>ADLGSPCGGRLNSKDAGYITSPGYPQDYPSHQNCEWIVYAPEPNQKIVLNFNPHFEIEKHDCKYDFIEIRDGDSESADLLGKHCGNIAPPTIISSGSM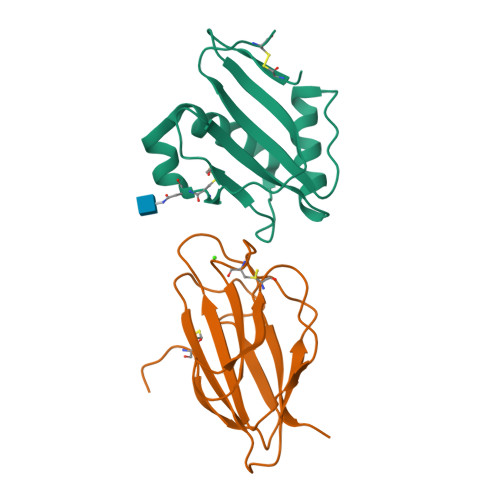LYIRFTSDYARQGAGFSLRYEIFKTGSGTHHHHHH[2x];>[2x]ADLGSHHHHHHGGMSLLSSIPMVSEQQHCIQHNHSSITFSLLTNKSDLEKCNFTRLQAVDRVIFDLFREFHHRVGDFPVTSDLKCSHNTSYRVIEYEVTKESLPRLQEAVSTLFPDLHLSEDRFLQIQAHDDKNCTGLH>MTMTLNELLATNPDGTLEDIAGKYNTSLFAVVEALPTAQCTLATGDRFDQVWDTIATWGEVTLISHTADAILEFKSELPTGTHRHGYFNLRGKNGLSGHIRATSCQHIAFIERKFMGMDTASVVFFNANGAAMFKIFLGRDSHRQLLSAQVDAFRALASELQPEQV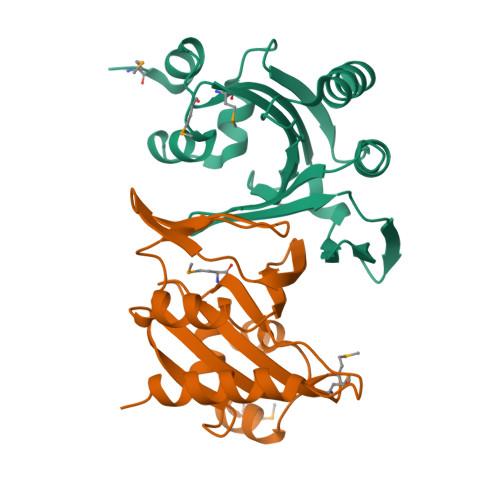LEHHHHHH[2x]4-({[4-(BUT-2-YN-1-YLOXY)PHENYL]SULFONYL}METHYL)-1-[(3,5-DIMETHYLISOXAZOL-4-YL)SULFONYL]-N-HYDROXYPIPERIDINE-4-CARBOXAMIDE 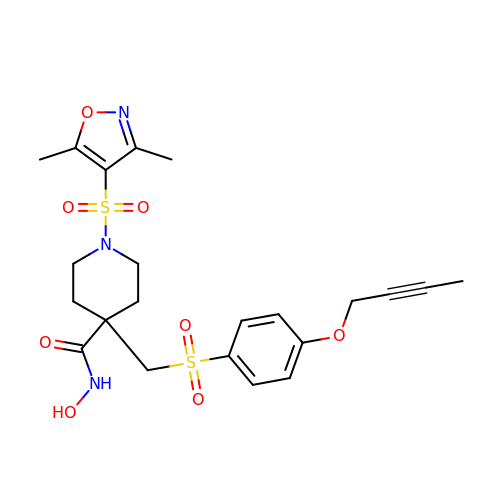| C22 H27 N3 O8 S2 | BIGQJQKSDHOEOM-UHFFFAOYSA-N>[12x]GPLGSMFHVRYRMEASCLELALEGERLCKSGDCRAGVSFFEA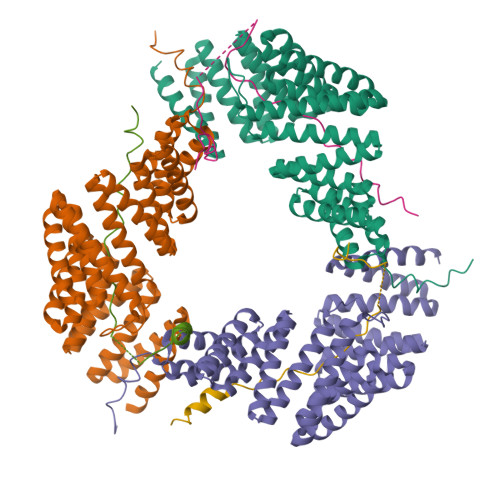AVQVGTEDLKTLSAIYSQLGNAYFYLHDYAKALEYHHHDLTLARTIGDQLGEAKASGNLGNTLKVLGNFDEAIVCCQRHLDISRELNDKVGEARALYNLGNVYHAKGKSFGCPGPQDVGEFPEEVRDALQAAVDFYEENLSLVTALGDRAAQGRAFGNLGNTHYLLGNFRDAVIAHEQRLLIAKEFGDKAAERRAYSNLGNAYIFLGEFETASEYYKKTLLLARQLKDRAVEAQSCYSLGNTYTLLQDYEKAIDYHLKHLAIAQELNDRIGEGRACWSLGNAYTALGNHDQAMHFAEKHLEISREVGDKSGELTARLNLSDLQMV;>GPLGSPDYGNSALLSLPGYRPTTRSSARRSQAGVSSGAPPGRNSFYMGTCQDEPEQLDDWNRIAELQQRNR[12x]[(2R,3R,4R,5R)-5-(6-AMINO-9H-PURIN-9-YL)-3-HYDROXY-4-(PHOSPHONOOXY)TETRAHYDROFURAN-2-YL]METHYL 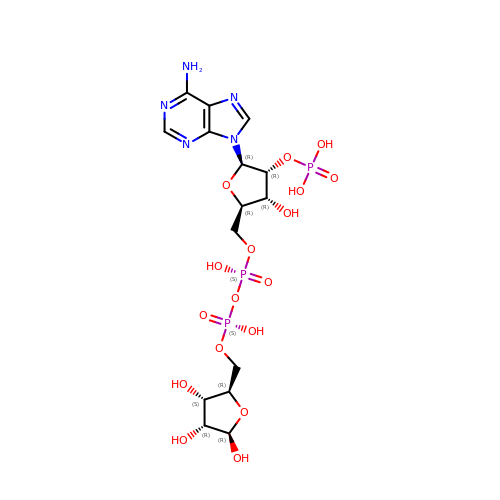[(2R,3S,4R,5R)-3,4,5-TRIHYDROXYTETRAHYDROFURAN-2-YL]METHYL DIHYDROGEN DIPHOSPHATE | C15 H24 N5 O17 P3 | ICNHOLCERMYLRZ-KEOHHSTQSA-N> 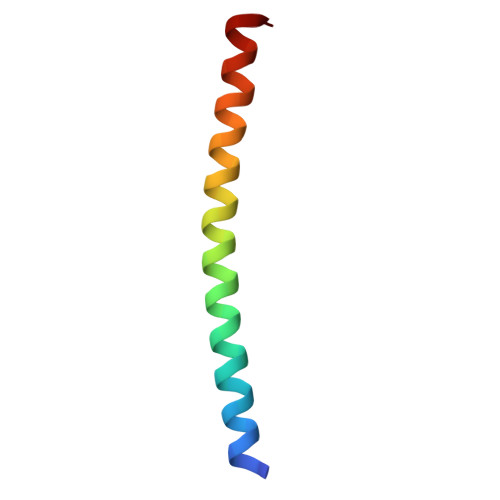XRMKQIEDKIEEIESKQKKIENEIARIKKLLQLTVWGIKQLQARIL>MGSSHHHHHHSSGRENLYFQGHMKTVLAFGDSLTWGADPATGLRHPVEHRWPDVLEAELAGKAKVHPEGLGGRTTCYDDHAGPACRNGARALEVALSCHMPLDLVIIMLGTNDIKPVHGGRAEAAVSGMRRLAQIVETFIYKPREAVPKLLIVAPPPCVAGPGGEPAGGRDIEQSMRLAPLYRKLA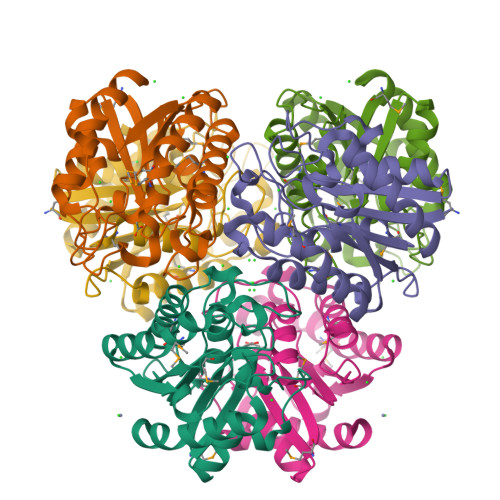AELGHHFFDAGSVASASPVDGVHLDASATAAIGRALAAPVRDILGS[3x]(2S)-butane-1,2-diol 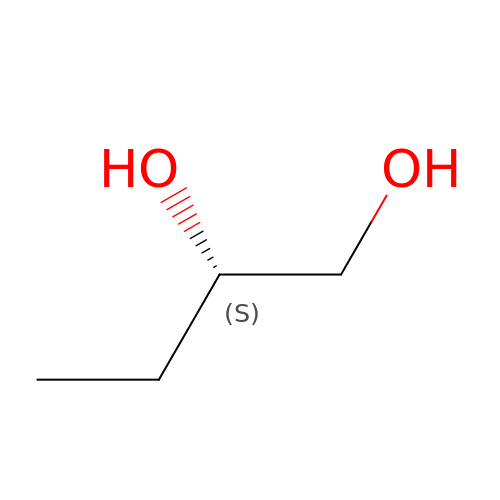| C4 H10 O2 | BMRWNKZVCUKKSR-BYPYZUCNSA-N> GRQGKTL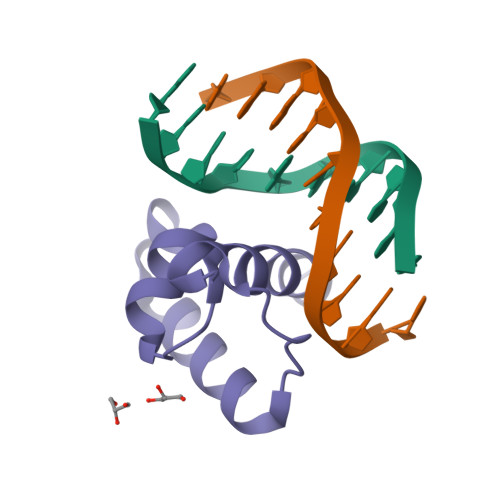KRPRLVWTPQLHKRFVDVVAHLGIKNAVPKTIMQLMNVEGLTRENVASHLQKYRLYLK Here, we show that the R-SNAREs VAMP8, VAMP3, and VAMP2, which cycle between the plasma membrane and endosomes, bind directly to the ubiquitously expressed, PtdIns4,5P2-binding, endocytic clathrin adaptor CALM/PICALM. X-ray crystallography shows that the N-terminal halves of their SNARE motifs bind the CALMANTH domain as helices in a manner that mimics SNARE complex formation. In this study, we provide structural, biochemical and in vivo data to show that the internalization of VAMP8, and consequently that of the highly related small R-SNAREs, VAMP3 and VAMP2, is mediated by specific, direct interactions between the N-terminal halves of their SNARE motifs and the ANTH (AP180 N-terminal Homology) domain of the endocytic clathrin adaptor CALM. Thus, CALM:R-SNARE interactions ensure that R-SNAREs, required for the fusion of endocytic clathrin-coated vesicles with endosomes and also for subsequent postendosomal trafficking, are sorted into endocytic vesicles.

If this hydrophobic trough were indeed the VAMP binding site on CALMANTH, then deletion of helix 11 would be expected to increase VAMP8 binding. However, a truncated CALMANTH construct missing helix 11 and the preceding ten residues, termed CALMANTH(1-264), unexpectedly showed no binding to VAMP8 by GST pull-down experiments and ITC while still displaying normal binding to PtdIns4,5P2 containing liposomes by SPR (data not shown). Multiangle light scattering (MALS) indicated that in solution CALMANTH(1-264) is in fact a tight dimer. This was confirmed by the determination of the structure of CALMANTH(1-264) at 1.7Å resolution (final R/Rfree 0.170/0.191). The dimeric structure explained the lack of VAMP8 binding since the dimer interface (burying 2100Å2 of accessible surface area in total) was the proposed VAMP8 binding site. As there were no other significant changes between the surfaces of CALMANTH and CALMANTH(1-264), these data strongly indicated that the hydrophobic trough in which helix 11 (when formed) sits was indeed the VAMP8 binding site on CALMANTH.

>GSPIGIHMSGQSLTDRITAAQHSVTGSAVSKTVCKATTHEIMGPKKKHLDYLIQCTNEMNVNIPQLADSLFERTTNSSWVVVFKSLITTHHLMVYGNERFIQYLASRNTLFNLSNFLDKSGLQGYDMSTFIRRYSRYLNEKAVSYRQVAFDFTKVKRGADGVMRTMNTEKLLKTVPIIQNQMDALLDFNVNSNELTNGVINAAFMLLFKDAIRLFAAYNEGIINLLEKYFDMKKNQCKEGLDIYKKFLTRMTRISEFLKVAEQVGIDRGDI[2x]>[2x]MGHHHHHHSGENLYFQGTMTLKEFIK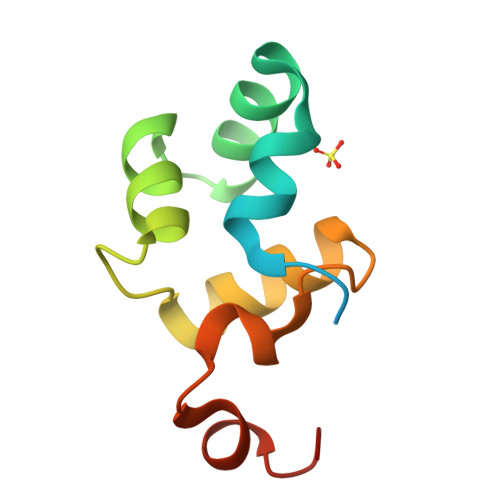SLRVGDAKKFAARLGVSPSYLSQMASGRTAISPTRALMIESATEGQVSRAELRPHDWELIWPEYASGI Pyruvate carboxylase (PC) catalyses the MgATP-dependent conversion of pyruvate to oxaloacetate. PC is a member of the biotin-dependent carboxylase family and contains biotin carboxylase (BC), carboxyltransferase (CT) and biotin carboxyl carrier protein (BCCP) components. On the other hand, in a diverse array of Gram-negative bacteria among the phyla Proteobacteria and Aquificae, the PC enzyme is encoded by two separate genes, with the BC domain residing in a 52 kD α subunit and the CT and BCCP domains in a 67 kD β subunit. We report here the structures of the two-subunit PC from Methylobacillus flagellatus (MfPC).

To improve the diffraction quality, we introduced three single-site mutations (K419A, E421A and E422A) in the β subunit designed to reduce the surface entropy. We then removed the flexible B sub-domain (residues 131–201) of the BC domain and replaced it with a Gly–Ser–Ser–Gly linker. A mutant protein having this deletion and the three single-site changes produced a different crystal form with better diffraction, allowing us to determine the crystal structure of the MfPC holoenzyme at 3.0 Å resolution using the molecular replacement method with the SaPC structure9 as the search model. Contrary to the expectations of an α4β4 holoenzyme, the structure revealed a 370 kD α2β4 oligomer for the MfPC mutant, with one BC dimer and two CT dimers. The mutant holoenzyme has overall dimensions of 140 × 130 × 70 Å and adopts a shape similar to the letter U, strikingly different from the holoenzyme architecture of single-chain PCs. The BC dimer forms the bottom and a CT dimer is on each arm of the U shape, leaving a large cavity in the middle. Of the three BCCP domains that are observed in this mutant holoenzyme, two are situated between the BC and CT domains, near the bottom of the U-shaped structure. The third BCCP domain is located in the active site of the distal β subunit with good electron density (β2), and its biotin is well ordered, but it comes from a proximal β subunit (likely β1). Therefore, the BCCP domains are extensively swapped in the holoenzyme. The proximal CT domain active site is accessible to BCCP in the mutant structure, but inaccessible in the wild-type structure due to clashes with the BC dimer.

>[2x]MIKKILIANRGEIAVRIVRACSEMGIKSVAIYSDADRHALHVKKADEAYNIGSDPVLGYLNAHNIVNLAVASGCDALHPGYGFLSENPELAEICARRGIKFIGPDAKVIRQMGDKIQARTAMIKAGIPCVGSSGVVNPRHIEVQVLADSHGNVIHLFERDCSIQRRNQKLIEIAPSPQLSKAQREYIGNLAVKAAKAVGYKNAGTVEFLLDSDNNFYFMEMNTRLQVEHTVTEQITGIDIVQEQIRVADGQRLQYKQSEVQYRGFAMEFRINAEDPKNDFLPSFGKITRYYAPGGPGIRMDAAMYSGYVIPPYYDSMCAKLTVWALNWESVVERGRRALNDTVVYGVKTTIPYYQEILKHPDFRNAIFNTSFVESHPELANYATQFPRELVAAAISAAIAAHEGI;>[4x]MAKVHVTDVVLRDGHQSLIATRMRTDDMLPICSKLDAVGYWSLEAWGGATFDACVRYLREDPWERLKKLRKALPNSRLQMLLRGQNLLGYRHYSDDVVRAFVQKSADNGIDVFRIFDAMNDLRNLKVSIESVKAVGKHAEGTISYTTSPVHDIPYFVNLAKELESFGCDTIAIKDMASLLTPQVTGDLVKALREAVSLPIHLHAHATSGLASMSIQRAVDNGVAIVDGCISSFAEGASLPATESIVAALKGTEYDTGLDIGLLQEISAYFREVRKKYWQFESEFTGVDTRVLVNQVPGGMISNLSNQLKEQGALDRMDAVLDEIPRVREDLGYPPLVTPTSQIVGTQAVLNVMTGARYKSVTNEVKNYLLGHYGKAPSTVNPDVRNLAVGNAQVIECRPADLLTAEMEKLRNEVEGLAASAADVLTYAMFPDLAKTFLQERNAGSLKPEPLLDKEAVTSRESHSRFAPTEFNVTLHGETFHIKLTGSGHHGEEQRPFYVSVDGVTEEVVVEILNEIEVSGGGQSSGEAKRKASSAASSGRPRPTHAGCVTTAMPGTIVDVKVNVGDKVSAGDAVLVIEAMKMENEIQASKSGVVVAINVKKGDSVTPDEALLEIQPD>[2x]MATHHTLWMGLALLGVLGDLQAAPEAQVSVQPNFQQDKFLGRWFSAGLASNSSWLREKKAALSMAKSVVAPATDGGLNLTSTFLRKNQCETRTMLLQPAG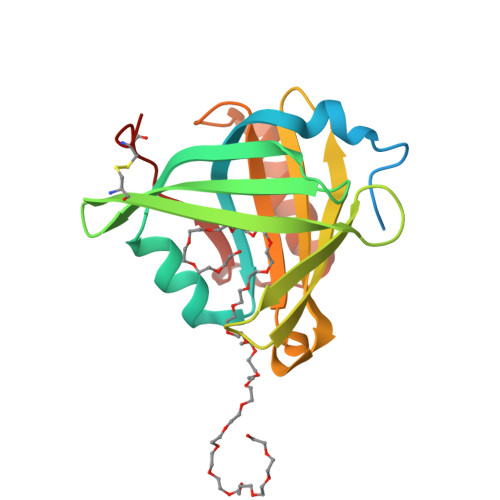SLGSYSYRSPHWGSTYSVSVVETDYDQYALLYSQGSKGPGEDFRMATLYSRTQTPRAELKEKFTAFCKAQGFTEDTIVFLPQTDKCMTEQ> GSMASLPVLQKESVFQSGAHAYRIPALLYLPGQQSLLAFAEQRASKKDEHAELIVLRRGDYDAPTHQVQWQAQEVVAQARLDGHRSMNPCPLYDAQTGTLFLFFIAIPGQVTEQQQLETRANVTRLCQVT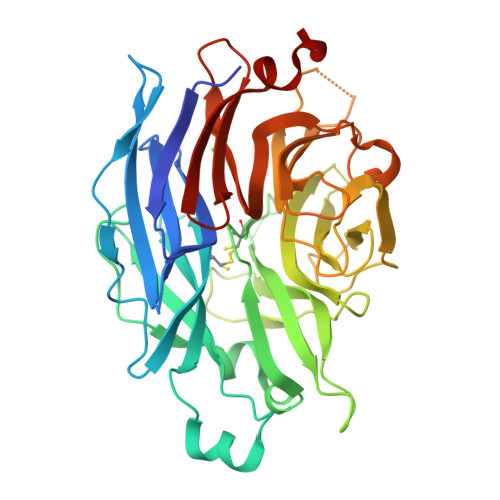STDHGRTWSSPRDLTDAAIGPAYREWSTFAVGPGHCLQLNDRARSLVVPAYAYRKLHPIQRPIPSAFCFLSHDHGRTWARGHFVAQDTLECQVAEVETGEQRVVTLNARSHLRARVQAQSTNDGLDFQESQLVKKLVEPPPQGCQGSVISFPSPRSGPGSPAQWLLYTHPTHSWQRADLGAYLNPRPPAPEAWSEPVLLAKGSCAYSDLQSMGTGPDGSPLFGCLYEANDYEEIVFLMFTLKQAFPAEYLPQ Topoisomerase III (TOP3) is a member of the type IA topoisomerase family, which functions mainly in relaxing the supercoiled DNA and in resolving recombination intermediates during meiosis and DNA repair. TOP3β is an atypical topoisomerase that can recognize both DNA and RNA as the substrates12132223242526. Eukaryotic TOP3α and β are unique in that they interact with their specific auxiliary factors, RMI1 and TDRD3, respectively, and coexist with them in the cell. We determined the crystal structures of human TOP3β TOPO domain, TDRD3 DUF1767 and OB domains (DUF–OB) and their complex at 3.44 Å, 1.62 Å and 3.6 Å resolutions, respectively.

The TOPO domain of TOP3β exhibits a toroidal-shaped structure, which is characteristic of the type IA topoisomerase. The TOPO domain is further divided into four subdomains (domains I–IV). The cavity formed by domains I, III and IV constitutes a Mg2+-bound catalytic pocket, where the catalytic residues are spatially arranged in a manner similar to those of other type IA topoisomerases. Previously reported E. coli TOP3 structures showed a transition from a closed conformation to an open conformation in the type IA enzyme upon binding of the substrate DNA39. Our substrate-free TOP3β structures adopted the closed conformation. Domain II of TOP3β appears more flexible than domains I, III and IV in the present TOP3β structures (one from the complex and two from the apo TOP3β in the asymmetric unit), indicative of its intrinsic flexibility for the induced fit binding to TDRD3. The R472Q mutation of TOP3β, which is located in domain II, has been found in schizophrenia patients. The R472Q mutation may hardly affect the tertiary structure of TOP3β, as the side chain of Arg472 is exposed to the solvent and partly disordered. However, the substrate-binding cavity of TOP3β is similar to that of TOP3α. We could find no TOP3α- or TOP3β-specific structural element that could determine their substrate preferences.

>[2x]PGHMKTVLMVAEKPSLAQSIAKILSRGSLSSHKGLNGACSVHEYTGTFAGQPVRFKMTSVCGHVMTLDFLGKYNKWDKVDPAELFSQAPTEKKEANPKLNMVKFLQVEGRGCDYIVLWLDCDKEGENICFEVLDAVLPVMNKAHGGEKTVFRARFSSITDTDICNAMACLGEPDHNEALSVDARQELDLRIGCAFTRFQTKYFQGKYGDLDSSLISFGPCQTPTLGFCVERHDKIQSFKPETYWVLQAKVNTDKDRSLLLDWDRVRVFDREIAQMFLNMTKLEKEAQVEATSRKEKAKQRPLALNTVEMLRVASSSLGMGPQHAMQTAERLYTQGYISYPRTETTHYPENFDLKGSLRQQANHPYWADTVKRLLAEGINRPRKGHDAGDHPPITPMKSATEAELGGDAWRLYEYITRHFIATVSHDCKYLQSTISFRIGPELFTCSGKTVLSPGFTEVMPWQSVPLEESLPTCQRGDAFPVGEVKMLEKQTNPPDYLTEAELITLMEKHGIGTDASIPVHINNICQRNYVTVESGRRLKPTNLGIVLVHGYYKIDAELVLPTIRSAVEKQLNLIAQGKADYRQVLGHTLDVFKRKFHYFVDSIAGMDELMEVSFS> GSKRFSDIPQTIDIPMQDDVEVEIDLQVLPDDPTELCSVFENEQSPRIYWMTVALAYAKQNKIDFAIEMLLRGANVLQGNQREKLGIITCICWLYLWKSREAPRVAPDGVPASEAKTKEYYLQLATQSLNDASRINPAFPPLFLARGVLILLKASLQPSSKAPGAVDSNKAEQLRNALKSFEEAIRVSQGRNMLAVMGKARALFSLGRYPESLAAYQDVVAKMPDMVDPDPRIGIGCCFWQLGFKDDAKIAWERCLEINPDSKHANILLGLYYLDASGHVPTNSPEFIRLYKKAMTEYTQKSFKLDKNLPLTCATFAGYFLSRKQFGNVDALAHKAIQYTDVNAIASDGWYLLARKEHYDGNLERASDYYRRADDARGGAERGYLPAKFGAAQLSVLKNDLGEAKLRLEKMIQHSKNYEAMILLGTLYAEEVFANQSAAVKEDKSAEAKKAISLLEGVRSAWKDPKRNLSPDAAVLLNLARLYESESPDKALQCLQQVEQLEIDQIPQSEYPPDAEDEAAARAAIRKLLPPQLLNNIGCFYSQEGKHRLATEFFQAALDSCARISQTENDLDI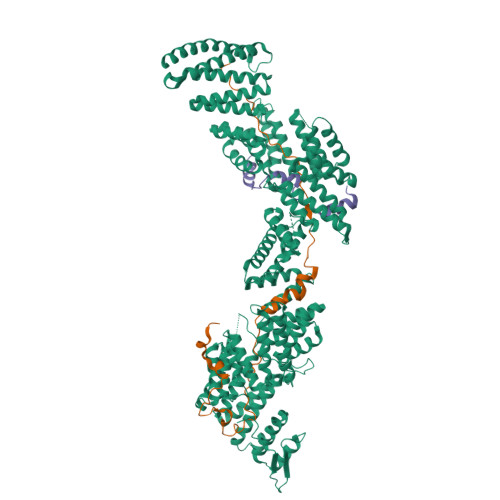DALLTTIPFNLGRSYEYEGDIDKAIETYEQLLSRHSDYTDARTRLAYIKLRRNPNKEGPDAVAKLYQENPSDLEVRGLYGWFLSKVNSKKRPANIAEDPEQRHYKHTLQSYDKHDRYALVGMGNLHLMAAREMRRETEQDRQKRSAAYNRAVEFFDKALQLDPKNAYAAQGIAIALVEDRKDYKNALQIFIKVRETIQDAHVYVNMGHIYAELRQFSKAIESYEIALSKEGKANDAGIISCLGRTWLNKGRAERNLDAYKMALDQAKKAVAVAPDQLHFKFNVAFVQIQIALVLHSMRESERNSFQLEEAAEGLEEAIKILDEIAASPSPPYPRHDIEQRANMARNTQRKQLERALASQREYEAKN;> SAASGRAGRGTLDPRLAQIYSGERRMGDRNTALRGIKPTDFSHVRKLAAPFVTRKPGAAPSAGVGASATLALNQ;> SMSSSQSRSGGERMIHQDYIARIRYSNALPPPPIPPKLLDIPNTGLASGQYTAPGFASRLAREQPLNIEADAELGMPLDLVGMPGVFDGDESSIQAPAQPPPVHPHDRPLLRPLSTLGKPK>SNAMNRLKNMSKYSDAKELASLTLGKKTEYANQYDPSLLQPVPRSLNRNDLHLSATLPFQGCDIWTLYELSWLNQKGLPQVAIGEVSIPATSANLIESKSFKLYLNSYNQTRFASWDEVQTRLVHDLSACAGETVTVNVKSLNEYTAEPIVTMQGECIDDQDIEIA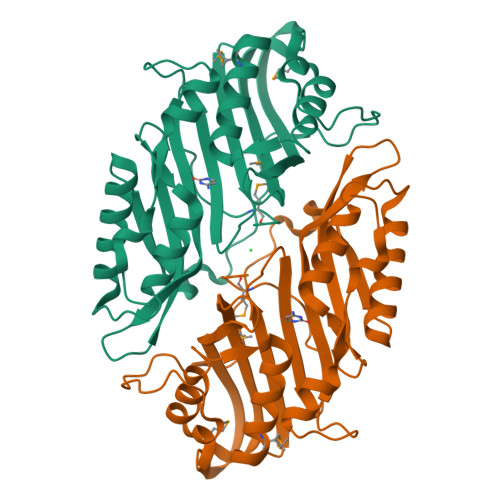NYEFDDALLQGAAQGEEVSEVLHSHLLKSNCLITNQPDWGSVEIAYHGAKMNREALLRYLVSFREHNEFHEQCVERIFTDIMRYCQPQSLTVYARYTRRGGLDINPFRSSHQSAPNHNQRMARQ[2x]>[2x]GPLPAHDASKVRASGPGLNASGIPASLPVEFTIDARDAGEGLLTVQILDPEGKPKKANIRDNGDGTYTVSYLPDMSGRYTITIKYGGDEIPYSPF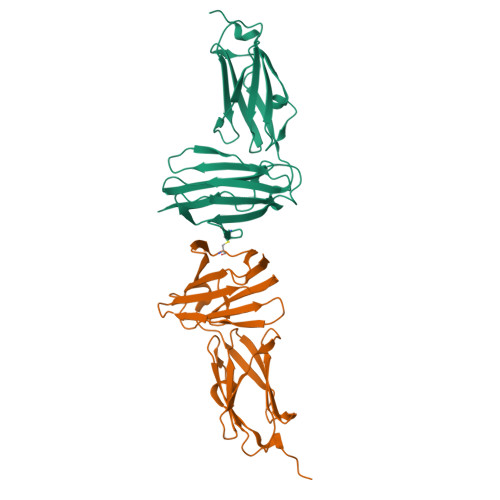RIHALPTGDASKCLVTVSIGGHGLGACLGPRIQIGQETVITVDAKAAGEGKVTCTVSTPDGAELDVDVVENHDGTFDIYYTAPEPGKYVITIRFGGEHIPNSPFHVLATE>[5x]MYFFSVDPRNGASKSGDVCGSCCCESISARPGEVNGVMVSYAAWSAPLRGHGLTNKTTFEIDGVSVTPPKVSNAFGRTKVGVVFEGTLSDLFPNPEGEQVEYEISELNGPSNGVVELGANGAFTYTPGALFTGVDRFWFSINGNIGEYVISVDPTTSELPQPPFTTPVYVPAARRSVDPRTHVLKFVLGVSPAAIPGDVYRLTVRQVAIDCDGNEFVHISCYDISIGSCG;>METKLTYGNRVTLPEFAKYIVAPAFHEIEGRAIPVTGVDDDASGTQATKLPFVLVGLRQGDTSGPATIAGNSTINLRDDFIVEFNMKKERYRDRKGGETPFFSYYDYESIRDRLFNSMIEFSGEHGITFEFVSLDISTEGDVVYIEFRFRQNYEWCETVREADTTIEAGRFSINLQGC[2x];>MACNKQNGVKNILITFTDCDTQEVIGPISHEQPDDTLPTYKNCAWTN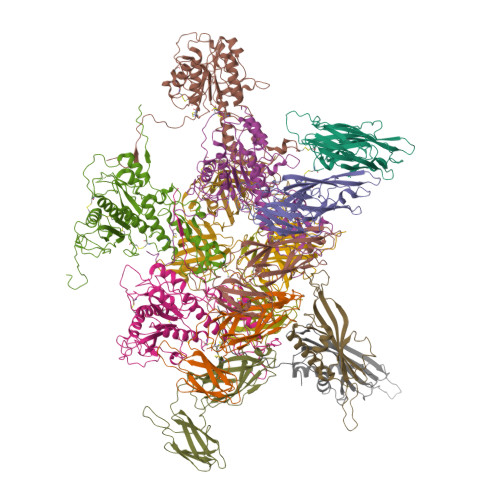TALTNGYVQRSASNATMTLPVVRDLRVPLAFYQGCAQVDVQVEKFDGTVMTLTEGAVVEPEESDGRSVTMNIVASEIDELLPPGSLAAA[4x];>MAQDALSDGFVRLCIDPSLNFFGEGCKILVEGQMTDDGSATPDAVTCVTSELDIIERFGQGSVLTESLRKVFCTCKSGVSVYALPREDAAAGVKAVYTLTIAGPATTDGRVQLYMGEAEYAVDIGVDAGDTATDIAAAIVAAISPDFPYAATAAAGVITLTARNAGTIGNHLSVIYTNLGSCTSVTPEGVTVTFAQTTAGSVNPTPNDYATVVNECCFAVYVLSSDDTDWQENLRDWIRSAWDCSKPQCFGHGYVFNKGTLGQVLADGDNSAELSRLALPTTYPVLPYLTNAAYGALSACSTCNNPELNIQGQTFGLLSCINMPESCTPGWTFGEVTQLQANGFVVSGPSTTSGQGNYTSPYIYNDVTNYLRDEKNRPNATFRDASSRRLAAATGVALAEFLQQFNGLAVFTKNTNIRTGIIGTNPRLMLGKIRKWAQDNVGTLFSEFDNINEDIQLLTDFEVQPKCVGQPGIFHLNMRYRPPVRGARINVNMAPALFDNCDR[4x]> MNPFQKNESKETLFSPVSIEEVPPRPPSPPKKPSPTICGSNYPLSIAFIVVNEFCERFSYYGMKAVLILYFLYFLHWNEDTSTSIYHAFSSLCYFTPILGAAIADSWLGKFKTIIYLSLVYVLGHVIKSLGALPILGGQVVHTVLSLIGLSLIALGTGGIKPCVAAFGGDQFEEKHAEERTRYFSVFYLSINAGSLISTFITPMLRGDVQCFGEDCYALAFGVPGLLMVIALVVFAMGSKIYNKPPPEGNIVAQVFKCIWFAISNRFKNRSGDIPKRQHWLDWAAEKYPKQLIMDVKALTRVLFLYIPLPMFWALLDQQGSRWTLQAIRMNRNLGFFVLQPDQMQVLNPLLVLIFIPLFDFVIYRLVSKCGINFSSLRKMAVGMILACLAFAVAAAVEIKINEMAPAQPGPQEVFLQVLNLADDEVKVTVVGNENNSLLIESIKSFQKTPHYSKLHLKTKSQDFHFHLKYHNLSLYTEHSVQEKNWYSLVIREDGNSISSMMVKDTESRTTNGMTTVRFVNTLHKDVNISLSTDTSLNVGEDYGVSAYRTVQRGEYPAVHCRTEDKNFSLNLGLLDFGAAYLFVITNNTNQGLQAWKIEDIPANKMSIAWQLPQYALVTAGEVMFSVTGLEFSYSQAPSSMKSVLQAAWLLTIAVGNIIVLVVAQFSGLVQWAEFILFSCLLLVICLIFSIMGYYYVPVKTEDMRGPADKHIPHIQGNMIKLETKKTKL;> AF

PepT1 belongs to the solute carrier family 15 (SLC15), also known as the proton-coupled oligopeptide transporter (POT) family, which consists of four members in eukaryotes: PepT1 (SLC15A1), PepT2 (SLC15A2), PhT1 (SLC15A4), and PhT2 (SLC15A3). PepT1 and PepT2 are best characterized and mediate the uptake, distribution, and resorption of di- and tripeptides in the body. PepT1 and PepT2 are secondary active transporters, which are energized by the inward-directed electrochemical proton gradient. On a structural level, human PepT1 (HsPepT1) is 708 and human PepT2 (HsPepT2) is 729 amino acids long. Both polypeptides consist of a core transporter unit of predicted 12 transmembrane helices (TMs) of the major facilitator superfamily (MFS) fold and an extracellular immunoglobulin-like domain (ECD) placed between TM9 and TM10.

HsPepT2, on the other hand, has been trapped in a substrate-bound inward-facing partially occluded state. The HsPepT2 model is lacking the first 40 residues at the N terminus and the last 32 C-terminal residues, which are predicted to be disordered. Recombinantly expressed and purified HsPepT2 used for structure determination was stabilized against heat unfolding in the presence of the dipeptide Ala-Phe in a concentration-dependent manner, confirming substrate binding of detergent extracted HsPepT2. The N and C termini of the dipeptide are clamped by electrostatic interactions with N192, N348, E622, R57, and K161, respectively. The phenyl group side chain is accommodated in a hydrophobic pocket formed by Y94, W313, L316, W649, L650, and I653, referred to as the side-chain pocket. In the HsPepT2 structure, the cytoplasmic side ends of TM4 and TM5 in the N-bundle are in close proximity to TM10 and TM11 in the C-bundle, narrowing the exit route from the peptide binding site to the cytosol, although without fully closing it as instead was observed in outward-facing HsPepT1. In the upper part of the transporter unit, the interaction between Y94 in TM2 (Y64 in HsPepT1) and N657 (N630 in HsPepT1) is disrupted and replaced by an interaction between Y94 and K161 (TM4), restricting bending of TM2. Additional intrabundle contacts including Q319 (TM7)–N348 (TM8) and Q316–R322 (TM7)–E674 (TM12) further stabilize the partially occluded inward-facing state. Last, the interbundle salt bridge between R206 (TM5) and D342 (TM8), together with the polar interaction network around H87 involving TM2, TM7, and TM8, tightly seals the central cavity from the extracellular space. These interactions need to be disrupted so that the transporter can cycle back to the outward-facing state observed in HsPepT1.> GHMAPGQKECDNALRQLETVRELLENPVQPINDMSYFGCLDSVMENSKVLGEAMTGISQNAKNGNLPEFGDAIATASKALCGFTEAAAQAAYLVGVSDPNSQAGQQGLVEPTQFARANQAIQMACQSLGEPGCTQAQVLSAATIVAKHTSALCNSCRLASARTANPTAKRQFVQSAKEVANSTANLVKTIKALDGDFTEENRAQCRAATAPLLEAVDNLSAFASNPEFSSVPAQISPEGRAAMEPIVISAKTMLESAGGLIQTARALAVNPRDPPRWSVLAGHSRTVSDSIKKLITSMRDKAPGQLECETAIAALNSCLRDLDQASLAAVSQQLAPREGISQEALHTQMLTAVQEISHLIEPLASAARAEASQLGHKVSQMAQYFEPLTLAAVGAASKTLSHPQQMALLDQTKTLAESAL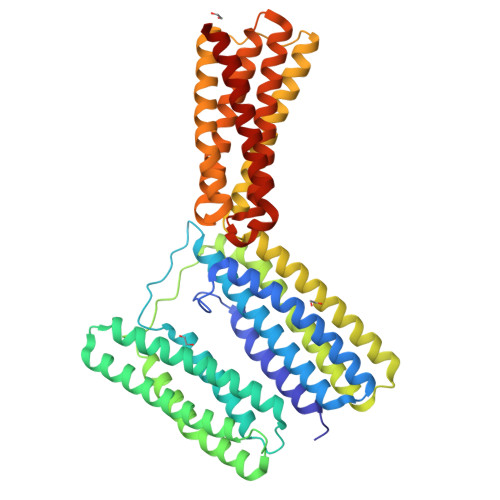QLLYTAKEAGGNPKQAAHTQYALYEAVYMMTEAVEDLTTTLNEAASAAG> TIKVGINGFGRIGRIVFRAAQKRSDIEIVAINDLLDADYMAYMLKYDSTHGRFDGTVEVKDGHLIVNGKKIRVTAERDPANLKWDEVGVDVVAEATGLFLTDETARKHITAGAKKVVMTGPSKDNTPMFVKGANFDKYAGQDIVSNASCTTNCLAPLAKVINDNFGIIEGLMTTVHATTATQKTVDGPSHKDWR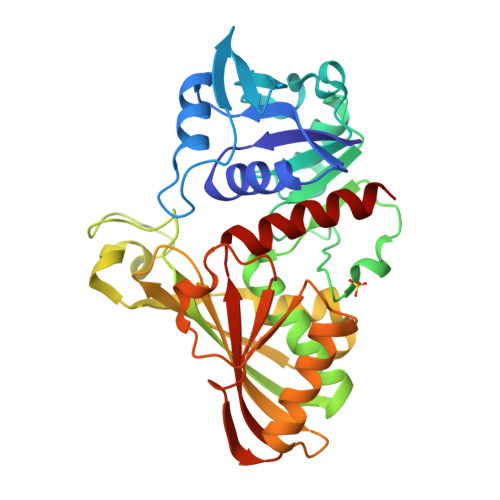GGRGASQNIIPSSTGAAKAVGKVLPELNGKLTGMAFRVPTPNVSVVDLTVRLEKAATYEQIKAAVKAAAEGEMKGVLGYTEDDVVSTDFNGEVCTSVFDAKAGIALNDNFVKLVSWYDNETGYSNKVLDLIAHISK> MAYRPSETLCG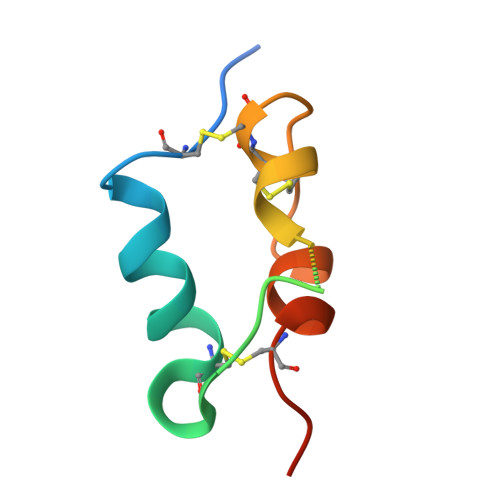GELVDTLQFVCGDRGFYFSRPASRVSRRSRGIVEECCFRSCDLALLETYCATPAKSE>[4x]MNGPKADIAWAASAEVANKPRLVFVGDELRYAQGANQRDVELDGFVNYHWLTSPGGLGLPKVMLEAGINAPAEVVGPDRSRRALIAIRSSPWKAGHETNPWHDEFDLDHGHVRYFGDHKPSTVGLPGETKGNRLLLEAARLHAGTTREERLLAPPLFLFRAVTVHRAGRAVVKGHVEFCGAAIIERLEHVVQRDPETGRSFPNLSLDLAVVSGGEI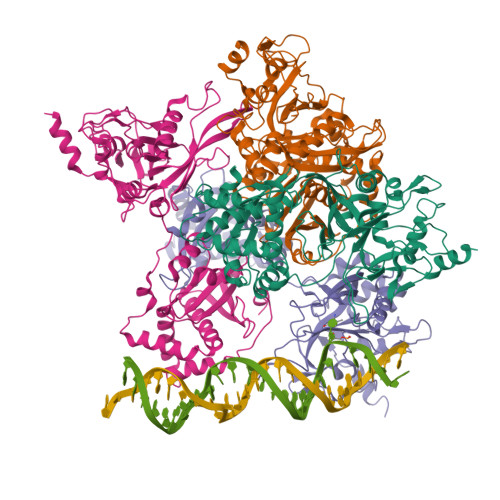DGVDFRWIDDRRNAALAAGETLRHAPESWIRWVRQGRLAIPGIRRRVLASAVQSSKEQQPASGSAEAATLQTLYKFYDGRKHAFELLASRVAAEVFRESGARYKEGWLSRSSGDGGVDFIGRIDMGSLKASTPVVVLGQAKCIQPTSSVSPEQVARVVARLRRGWIGVYVTTGSFSRQAQVEIIDDQYPVVLIAGGTLAATVRRMVQANYGGDLDALLASTVDEYGAAVTHRRPEEVISL> GPNYCFAGKTSSISDLKEVPRKNITLIRGLGHGAFGEVYEGQVSGMPNDPSPLQVAVKTLPEVCSEQDELDFLMEALIISKFNHQNIVRCIGVSLQSLPRFILLELMAGGDLKSFLRETRPRPSQPSSLAMLDLLHVARDIACGCQYLEENHFIHRDIAARNCLLTCPGPGRVAKIGDFGMARDIYRASYYRKGGCAMLPVKWMPPEAFMEGIFTSKTDTWSFGVLLWEIFSLGYMPYPSKSNQEVLEFVTSGGRMDPPKNCPGPVYRIMTQCWQHQPEDRPNFAI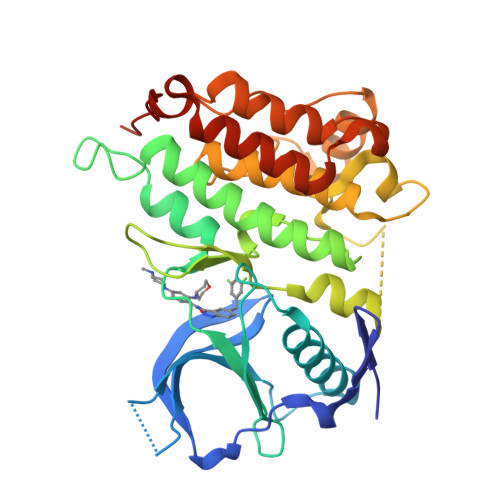ILERIEYCTQDPDVINTALPIEYGPLVEE> E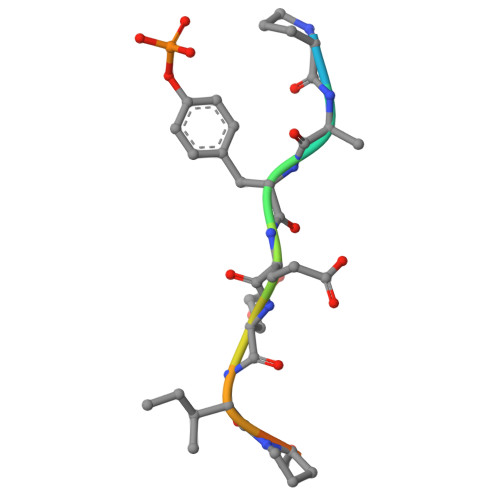PQYEEIPIYL> GASAPMVKIYTKNGDKGQTRIIGKQILYKNDP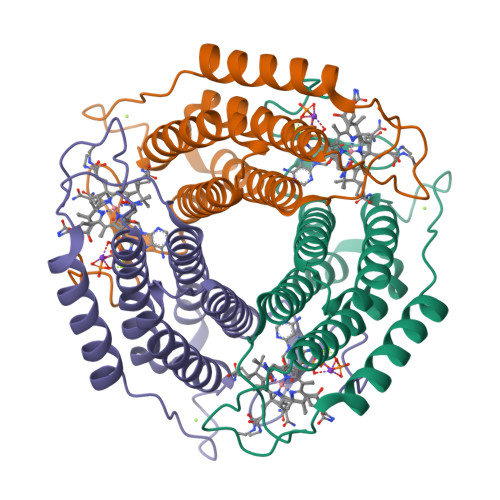RVAAYGEVDELNSWVGYTKSLINSHTQVLSNELEEIQQLLFDCGHDLATPADDERHSFKFKQEQPTVWLEEKIDNYTQVVPAVKKHILPGGTQLASALHVARTITRRAERQIVQLMREEQINQDVLIFINRLSDYFFAAARYANYLEQQPDMLYRNSKDVFR Carbonic anhydrases (CAs, EC 4.2.1.1) are metalloenzymes, which catalyze the reversible hydration of carbon dioxide. In order to learn more about the molecular mechanism of β-CA, we have determined the crystal structure of β-CA from Coccomyxa (Co-CA) in complex with five inhibitors: acetazolamide, thiocyanate, azide, iodide, and phosphate ions. Co-CA is a homo-tetrameric structure with one dimer present in the asymmetric unit. The catalytic zinc ion binds to the side chains of residues Cys-47, His-103, and Cys-106 in a tetrahedral geometry with the fourth ligand expected to be a water molecule in the native enzyme.

The structure of Co-CA in complex with acetazolamide, Co-CA-AZM, was refined at 1.9 Å. The maps show well-defined electron density for the entire acetazolamide molecule and for a neighboring glycerol molecule, both before and after refinement. The binding and orientation of AZM in Co-CA is similar to what has been observed in human CAII, and human CAI. The amide group of the sulfonamide part of the inhibitor is situated 2.0 Å from the zinc atom and positioned in a tetrahedral geometry. Furthermore, the amide group forms a hydrogen bond to the Oδ2 atom of Asp-49 (3.1 Å). The O1 atom of the sulfonamide group forms a hydrogen bond to the Nδ2 atom of Gln-38′ (3.0 Å), whereas the last oxygen of the group forms no hydrogen bonds but is in van der Waals' contacts with Val-71 and Ala-108. The direction of the inhibitor is restricted by its thiadiazole ring, which is sandwiched at the "channel gate". The two nitrogen atoms in the thiadiazole ring form hydrogen bonds to a water and a glycerol molecule, respectively. The nitrogen of the N-acetamido group forms a hydrogen bond to a water molecule, whereas the acetamido group itself is buried in a rather hydrophobic part of the active site cleft. The Ki of acetazolamide binding to Co-CA is 1 µM, which can be compared to the Ki values of acetazolamide binding to human CAII, human CAI, and pea CA with 0.01 µM, 0.2 µM, and 28 µM, respectively.

>MSAKDTADLSPLLEANRKWADECAAKDSTYFSKVAGSQAPEYLYIGCADSRVSPAQLFNMAPGEVFVQRNVGNLVSNKDLNCMSCLEYTVDHLKIKHILVCGHYNCGACKAGLVWHPKTAGVTNLWISDVREVRDKNAAKLHGLSADDAWDKMVELNVEAQVFNVCASPIVQAAWARGQPLSVHGIVYTPGTGLVKELIKPITGMEDAGALLRADLKQHCFFSESLA[2x]> MIIIRYLVRETLKSQLAILFILLLIFFCQKLVRILGAAVDGDIPTNLVLSLLGLGIPEMAQLILPLSLFLGLLMTLGKLYTESEITVMHACGLSKAVLIKAAMILAVFTGAVAAVNVMWAGPWSSRHQDEVLAEAKANPGMAALAQGQFQQASDGNAVMFIESVNGNRFHDVFLAQLRPKGNARPSVVVADSGELSQQKDGSQYVTL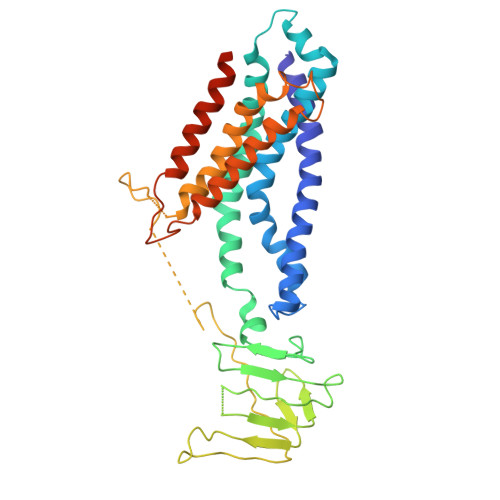NKGTRFEGTAMLRDFRITDFNNYQAIIGHQAVSADPDDTEQMDMRTLWKTHTDRARAELHWRFTLVATVFIMALMVVPLSVVNPRQGRVLSMLPAMLLYLVFFLLQTSIKSNGGKGKMDPAIWMWAINLLYFALAVLLNLWDTVPMRRFRARFNKGAA> MSDKLTRLERLNKEVKKQNKLKQHSKNNRFDDDMDIEAYEDDEQIEEDDFIDDTQEDKKYKKKYREIEDEFDQEIEEEEELNKKKKTKNTILNYTNTTAVTNNKKKAISKQIPDIDIEEIMKLTERKKKIEQEEAQLLQEEQELLEQEKREEEEKKRISQEAKSILREDCASSKTANSSKGKVDQNILNAINRDFSDDSNTVDSISEFQKLKSLAQKANLANESLKQSKVSNTEINLTNLSISQVKKINDYKNEDGSVDAYLYDYFYDAQVKPDKIYAFAKVQNKQTNAFDT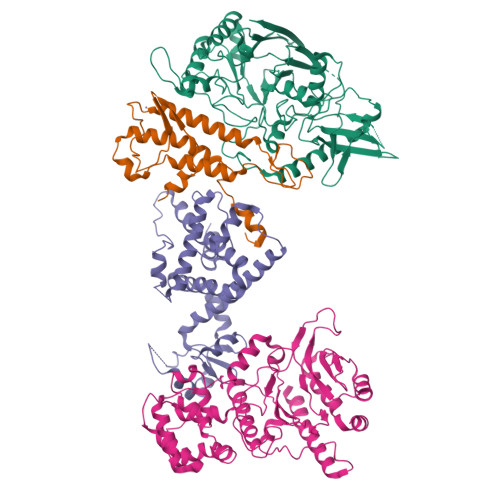CVIQIDTIIRNLFFYPSSDTVTEQQIKNEIAELLKKEQTSRKNVEFLGAFVDKNYAFELPIPRGKSRWYQVVMSYEYEVISPDTKGQYFSYCVGSTYSALETFLITKKITGPSWVRFQNVKDTTSCITNRKLEFRVDYTNQSNIQVLQKQLPTPPLSVVCISLKTSQQIVLSQKKKEYKKEIFNLNMKYHEGINIDNSNKDELNQFKSISFITHIDPTKKQDSITKKGTLPETTKFCLNELNLLEQFLVHFNEIDPDIVVAHDLYSTVFEIILTRIREKGIRKWNLLSKLINIGSSDIPKYGSSTFKTKMAMKGRLLVDTLLSSQEFVNCVEYTLEALAQKLFKIEIPRIDAKAYQQKFATYKLLNSLVDDTYQDIDYALRIMYHLQIVPLTKQLTSICGNIWMGSLQNQRAERNEMLLLHKFNQLNYVYPDNFKNLPESYKKKHKNAQIRKQYEEDEDQAQGNKNPKKKENKYKGGQVFEPEKGLYNEYIVLLDFNSLYPSIIQEFNVCFTTCVRDPIPLEMQMAPFLGNKKAAIQYSKNQNTKENKMQDEDEEDNENEQIVQTHDVLPTIEVIKGIAPLPSILQYLVEQRKVVKNQIKGQKDPQVIETLDIKQKAFKLVANSMYGCLGFSSSRFYAMPLASFITAKGRHILFDSKKIVEDMGYSVIYGDTDSLMIKPGTNEFLEAVKTGLSIKIKVNSKYKKLQLDIDGVFKNMLLLKKKKYATLKVANWEEVKNTNAPEKLEKEIKGIDVVRRDWCQLSRDAGNKILEIILESKSSENMLDDIKKYLIQLNDDINQKNIKNSNYYITKRLTKRVDQYGEKNLPHVAVAQRSIQEKGIDPQTYVNQIISYIICKNEQSSRLVDKAYSPQEFITQSKSLEIDLQYYKRFQLFEPIKRMLEVIEGINLQEIASILEVHYSVQHVSQNNELNAENVLNLKSKRNQFLTSIPRVLVDCKKCDQTFLFLGILEENADAASILKCKCGNDIYIQLKNKIALVVKELIRNFEENAIQIDNEEFEYTHQISLVGKAKQQKMSSFTLNQKLLSIQAMFDITKEEQENTQKVTIEKIKTIKKTLDDLLSKSQYNNLNLSNIFTSFGLLK;> MEEFEKILEEIDSANLSQNAVQQLKQLIISNGILDDEQLMEKWLFQLEAIIYNSKQKFLEAQLMDFKKNVLNQDIKKPQNDNFKKIKESEVQKNIDIIKGDADLFTKASSAKKQTSTQQANNAAIDCEEQLRQQLGKESMLDPKRFSYNSNLPQVNFEKNQHQNSNNMTIVDLFEQYDPNKIPNYLTNNIDKIRKHLEQRILTFKIQNYSQFIVNGEQLINDVSSYSKTEEVKMVGRLISTENGFLNTTNLRIELNRNQYFDLVFENDFDFGNNVLFPNQIVMVKGIINEKEELVVSELITDHIKEITDEEHPKIDNLNQDESQLIMVAAGPFSTVMSTQYTSFDNILHVAKTKKVSTLILLGPFLDIKNEILKDGSIIINSKEYTFEQLQNSLFEKAVKELEGKTQIIIVPSTRDILSTDSIPQMSLEIKVSEHKNSIHSYSNPAYIDIDKLRVYIANSDVGMITLQNSLLDKKIPYMQQSRLTFKALMNQQNLYSIYPMRNPQDSQQILETVKLPNINDFDIPFDYQLEQYPHIIISPSSLPKFATKIYNTVVINPNYVIRDGSQAGNFAIITLFKDSDIPIHERTRVDLYCL;> MEIETVEVAPQQEEEFKLDYDLLEEYYRSYFPVSQMVQWLSYPQDGDDTYFTRREFSFTLQNEVYLRYQMYNSEREFKNALLQKVPEKIDIGAVYDRPGKKGDDIKAKEKEFVIDIDMTDYDHIRTCCSKAKICEKCWKFMRVACDLISKSLDEDFGFQHVLWVYSGRRGIHAWVCDKEIRKANDYTRASIIDYLNILVDNSIGSSYVKPSLLKMEKSHLIERNAMKQLNQKNDDLKAEKESEKVFVEIVLREQNLFMKKPEIILEFLAKRSENLSKEVEKEWKTLKTSEQRYEALKELVSSEDKKKTHYLLEELRIWLLYPRLDVNVSKSTNHLLKSPFCIHPKTGNVCVPFTTEEISTFDPFSVPNISTLTTEEGSSKMKNSLKIFNKFLENLKKDV;> MINNKQIQKIQQISKFQLKEYIEMQMQQHSLNKQIKEEERNYILLENAIDNSNIQGFQTIQEIVQLAMQRMKMIKEIIQEEPRFNLIDPLSKPNYNRIRVANKFITVAIPKSDPEYELKNKQQYAKEVLSHFLCKMAYAFYAEPETWLEFARAEAFILMDKLKSGQHHANFFSDENLKIKTISDELFKQAFPKIEATFSSIKIKKNDSEVEQINIKKDNFKMFKFIDHPSMLSNNDVVLHKGYIIIYKESTSKIVQNIFIERLLDEMRLLQLKFQNNGSKLDDDRLSFLKDLHKAEIFNDSTQFNSTQIHHYELDRLAKRDMPACMTYLMYGLNQKLHLKHFGRLQLGLFLKGAGLSLNEALTFWQKKFSKTSADDFKKKYDYNIRHNYGKLGKQLDYTPMSCQKIIGFQPLKDEFHGCPYKTMESQQLKDFLKLSYNITDEQFVQVNIFKNQKQYQLACKEVFKVLNDTRDKTKEQFYPYFDKVGNHPNAYFEQSLRMHEPQRFQKQDEEKKQNKQNRNQNFSANKQSTNKNNQMDLEF> RSDSPEIPFQAAAGPSDGLDASSPGNSFVGLRVVAKWSSNGYFYSGKITRDVGAGKYKLLFDDGYECDVLGKDILLCDPIPLDTEVTALSEDEYFSAGVVKGHRKESGELYYSIEKEGQRKWYKRMAVILSLEQGNRLREQYGLGPYEAVTPLTKAADIS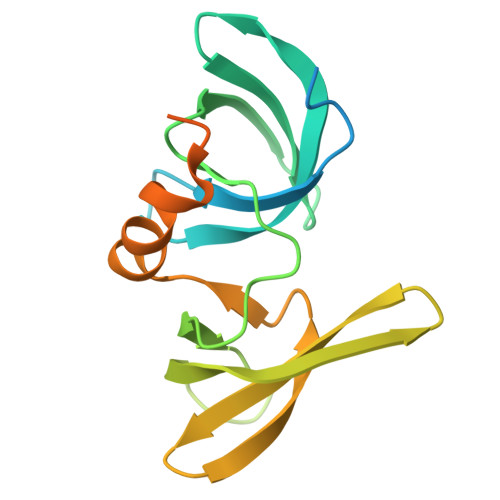LDNLVEGKRKRRSNVS> MFWLKTRIIEGEGSLSRLSREVKGHERVLILASGSMKRHGFLSEAEDYVKEAGAEVFSIAGLPAEPSVEVIEEFLPKVREFGPDLLVAMGGGSVIDTTKALKVFYDAPELNFGEIAFIDRFSKPKPVPRLKTLLIAIPSTSGAGSEVSGASVLKKGGVKYNIV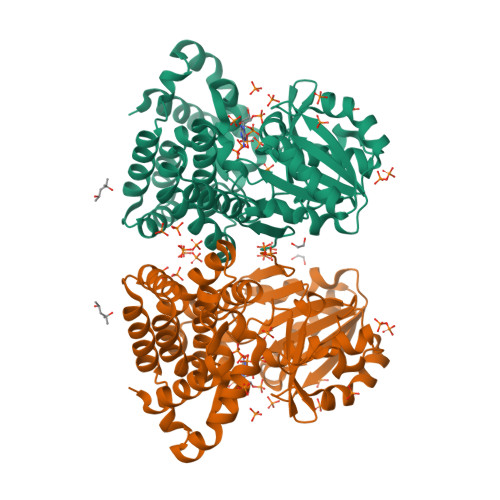TPEIAPDVAILDPRLPRTMPPEVARNSGLDVLVHGIEAYTTKVASPFSDAMAIKAIKTVYRWLPLSVKGDEEARARVHYAATMAGIAFLNARLGLCHAMSHKAAWIGPHGLLNAVFLPYVMEFNASKSDYARRRYAEIARELGFQTAKDLIEVVKELNEMLGVPKLGELVDEETFASKVEEMAEKTYHDGLIAFNPVEPKPEEIKELYLKAYRGE> GPGSMEASCLELALEGERLCKSGDCRAGVSFFEAAVQVGTEDLKTLSAIYSQLGNAYFYLHDYAKALEYHHHDLTLARTIGDQLGEAKASGNLGNTLKVLGNFDEAIVCCQRHLDISRELNDKVGEARALYNLGNVYHAKGKSFGCPGPQDVGEFPEEVRDALQAAVDFYEENLSLVTALGDRAAQGRAFGNLGNTHYLLGNFRDAVIAHEQRLLIAKEFGDKAAERRAYSNLGNAYIFLGEFETASEYYKKTLLLARQLKDRAVEAQSCYSLGNTYTLLQDYEKAIDYHLKHLAIAQELNDRIGEGRACWSLGNAYTALGNHDQAMHFAEKHLEISREVGDKSGELTARLNLSDLQMVLGLSYSTNNSIMSENT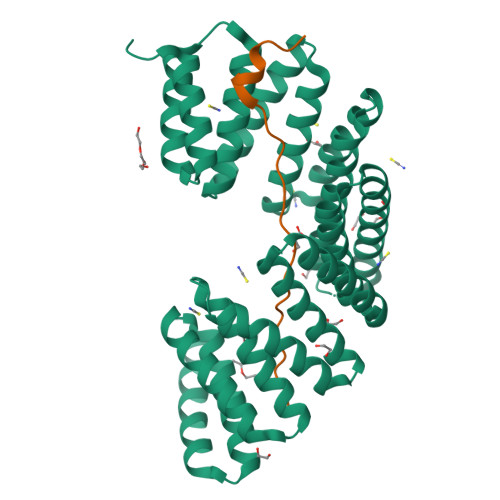EIDSSLNGVRPKLGRRHSMENMELMKLTPEK;> GPLGSDLPPKVVPSKQLLHSDHMEMEPETMETKSVTDYFSKLHMGSVAYSCTS(2-methyl-1,3-thiazol-5-yl)methyl 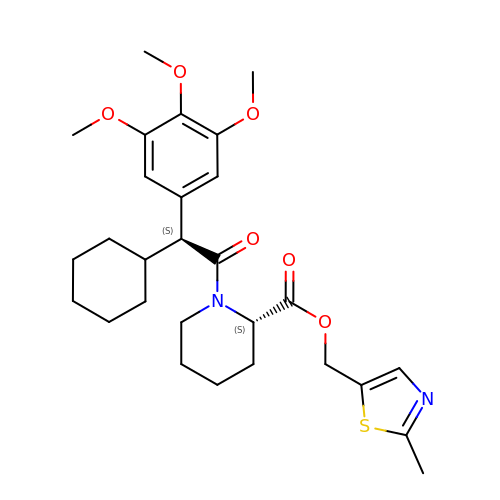(2S)-1-[(2S)-2-cyclohexyl-2-(3,4,5-trimethoxyphenyl)ethanoyl]piperidine-2-carboxylate | C28 H38 N2 O6 S | SVRWAJARXFNRPM-DHLKQENFSA-N Phosphoinositide-dependent protein kinase 1 (PDK1) is a master kinase that phosphorylates at least 23 AGC kinases at the activation loop, a site required for their activity. A linker connects the phosphoinositide-binding PH domain to the catalytic domain, which contains a docking site for substrates called the PIF pocket. PDK1 does not require binding to PIP3 to phosphorylate substrates such as S6K and SGK in vitro or in vivo. These phosphorylation events are mediated by a phosphorylation-dependent docking interaction between a C-terminal hydrophobic motif (HM) present in substrates and a regulatory site called the PIF-binding pocket (PIF pocket) in PDK1 (18, 24–33) (top). Here, we used a chemical biology approach to show that PDK1 existed in equilibrium between at least three distinct conformations with differing substrate specificities.

The angiotensin II type 1 receptor blocker valsartan inhibited PDK1 dimerization (IC50= 32 μM). Des(oxopentyl) valsartan did not disrupt PDK1 dimers, suggesting that the oxopentyl moiety was important for the interaction and disruption of PDK1 dimers. The effect of valsartan on WT PDK11-556 but not PDK11-556 [L155E] suggested that valsartan binds to the PIF pocket as well. In agreement with this prediction, valsartan but not des(oxypentyl)valsartan inhibited the interaction between His-PDK11-556 and biotin-PIFtide. To further understand the binding mode of valsartan, we crystallized PDK150-359 in complex with valsartan. We solved the high resolution structure of the PDK1-valsartan complex, which showed that valsartan binds to the PIF pocket of PDK1. Three molecules of valsartan produced a strong electron density at the PIF pocket and were modeled. Therefore, valsartan molecule #1, located on the helix α-B side of the PIF-pocket, could be responsible for disrupting PDK1 dimers. In such a model, valsartan molecule #1, which interacted with the helix α-B but also extended outwards, could act as a glue between the catalytic domain and the linker-PH domain to stabilize this conformation. Although PDK1 could bind HYG8 and PIFtide simultaneously, valsartan did not further enhance the temperature stability of the PDK1-HYG8 complex. These results are consistent with valsartan stabilizing a monomeric form of full-length PDK1 that is distinct from the monomeric form stabilized by HYG8 and functionally different because it does not bind PIFtide.

> GAMDGTAAEPRPGAGSLQHAQPPPQPRKKRPEDFKFGKILGEGSFSTVVLARELATSREYAIKILEKRHIIKENKVPYVTRERDVMSRLDHPFFVKLYFTFQDDEKLYFGLSYAKNGELLKYIRKIGSFDETCTRFYTAEIVSALEYLHGKGIIHRDLKPENILLNEDMHIQITDFGTAKVLSPESKQARANSFVGTAQYVSPELLTEKSACKSSDLWALGCIIYQLVAGLPPFRAGNEGLIFAKIIKLEYDFPEKFFPKARDLVEKLLVLDATKRLGCEEMEGYGPLKAHPFFESVTWENLHQQTPPKLT>NPAQFAQKTVLDEHVNDADIHVTATDKTNWNAKETVE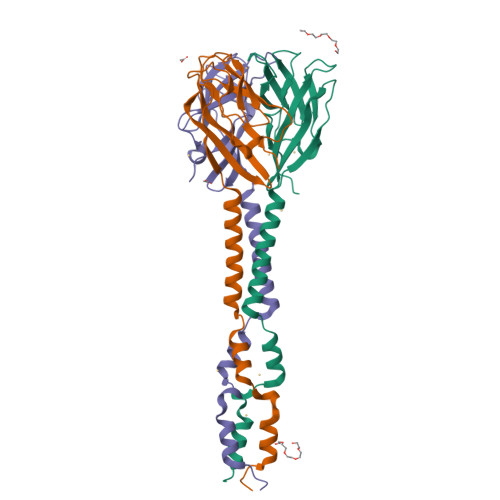GAQAKADKALADAKAFFELSSSVQSVTLTPKNGFVASQPLIARYIKFGNRFLVIVSGIVGKGTGSGTGICATLPTFLAPDASWNKLYSAAQQSTAASNQANIYLSVSADINIVGVGSVDVNTGLDGIIYLTKEVTT[3x]>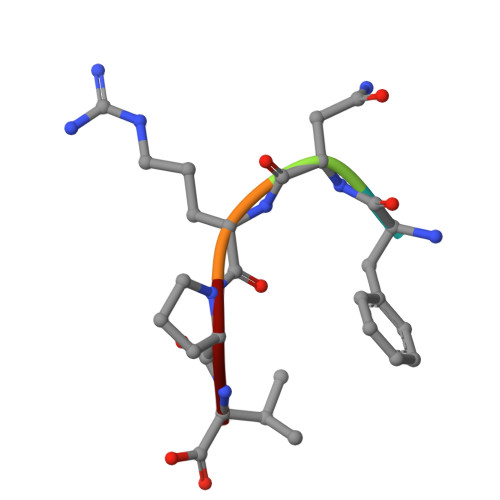 FNRPV Efflux pump antiporters confer drug resistance to bacteria by coupling proton import with the expulsion of antibiotics from the cytoplasm. Here, we uncover the proton-coupling mechanism of the Staphylococcus aureus efflux pump NorA by elucidating structures in various protonation states of two essential acidic residues using cryo-EM. NorA contains two essential membrane embedded acidic residues at positions Glu222 and Asp307 which are conserved across S. aureus strains and required for conferring fluoroquinolone resistance to the human pathogen methicillin-resistant S. aureus (MRSA). Hence, the two acidic residues serve as a “belt and suspenders” protection mechanism to prevent simultaneous binding of protons and drug that enforce NorA coupling stoichiometry and confer antibiotic resistance.

To determine whether protonation at Glu222 and/or Asp307 were responsible for triggering the conformational change to the inward-occluded state, we constructed the E222Q and D307N single mutants of NorA (NorAE222Q and NorAD307N). Remarkably, binding assays revealed each mutant bound FabDA1 at pH 5.0 and 7.5 with Kd values in the low micromolar range and neither bound to the outward-open-specific Fab36 at either pH value. Next, cryo-EM samples of NorAE222Q and NorAD307N in complex with FabDA1 were purified at pH 7.5, which we anticipated would induce deprotonation at Asp307 or Glu222, respectively. Following data collection and processing, we obtained cryo-EM maps at 3.35 Å resolution for NorAE222Q and 3.51 Å resolution for NorAD307N. Superimposition with wild-type NorA gave backbone Cα r.m.s.d. values of 0.73 Å for NorAE222Q and 1.07 Å for NorAD307N, as well as similar interfacial contacts with CDRH3 of FabDA1. Nevertheless, small but significant structural changes were observed within the substrate binding pocket for NorAD307N and NorAE222Q structures relative to NorA, providing clues into the proton-coupling mechanism of drug efflux. A similar trend was identified in the NorAE222Q structure, albeit to a lesser extent than in the NorAD307N structure. The nearest distances of Gln222 (mutant) to the backbone carbonyl of Phe140 and Asp307 to the side chain of Asn137 were ~1 Å longer than in the NorA structure. Furthermore, two rotamers of Asn137 were observed in the NorAE222Q cryo-EM map and were indicative of heterogeneity and a weaker interaction to Asp307 upon deprotonation. MIC values for the point mutants NorAE222Q and NorAD307N displayed substantial loss-of-function, nearly identical to the MIC value of MRSAΔnorA, which underscored their role in proton-coupled transport.

> MNKQIFVLYFNIFLIFLGIGLVIPVLPVYLKDLGLTGSDLGLLVAAFALSQMIISPFGGTLADKLGKKLIICIGLILFSVSEFMFAVGHNFSVLMLSRVIGGMSAGMVMPGVTGLIADISPSHQKAKNFGYMSAIINSGFILGPGIGGFMAEVSHRMPFYFAGALGILAFIMSIVLIHDPKKSTTSGFQKLEPQLLTKINWKVFITPVILTLVLSFGLSAFQTLYSLYTADKVNYSPKDISIAITGGGIFGALFQIYFFDKFMKYFSELTFIAWSLLYSVVVLILLVFANDYWSIMLISFVVFIGFDMIRPAITNYFSNIAGERQGFAGGLNSTFTSMGNFIGPLIAGALFDVHIEAPIYMAIGVSLAGVVIVLIEKQHRAKLKEQNMENLYFQGKLGPEQKLISEEDLNSAVDHHHHHHHHHH;> SVENHWYYFYWYMSP>[4x]SMKDHTEGLSDKEQRFVDKLYTGLIQGQRACLA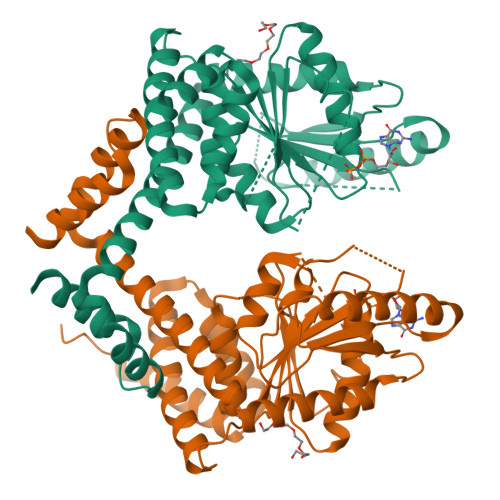EAITLVESTHSRKKELAQVLLQKVLLYHREQEQSNKGKPLAFRVGLSGPPGAGKSTFIEYFGKMLTERGHKLSVLAVDPSSCTSGGSLLGDKTRMTELSRDMNAYIRPSPTRGTLGGVTRTTNEAILLCEGAGYDIILIETVGVGQSEFAVADMVDMFVLLLPPAGGDELQGIKRGIIEMADLVAVTKSDGDLIVPARRIQAEYVSALKLLRKRSQVWKPKVIRISARSGEGISEMWDKMKDFQDLMLASGELTAKRRKQQKVWMWNLIQESVLEHFRTHPTVREQIPLLEQKVLIGALSPGLAADFLLKAFKSRD> MPPSKGLNGKLEKPKHALQAIVLSDSYNYRFRPLTLDKPRCLLPLANTPLIEYTFEFLALAGVQEVYVFCCAHAGQIREYIEKSKWNLPSSPFSVNTIVSRESLSVGDALRELDSKQLITSDFILVSGDVVSNVPLNEVLKEHRKRREDDKNAIMTMVVREASPFHRTRARTESSVFVIDKKTSQCVHYQANERGKHYVSMDPEIFNEHEELEVRNDLIDCQIDICSNDVPALFTENFDYQDIRKDFVYGVLTSDLLGKKIHCHVAKENYAARVRSLQTYDAISKDVLSRWVYPFVPDSNLLNQTFSYQRHQIYKEEDVVLARSCIIKARTLIGAYTKVG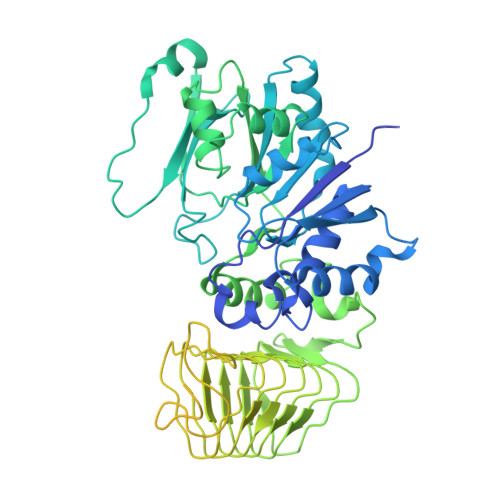DASVVANTIIGRNCTIGSNCSIDSAFLWEDVVIGDNCRIGKAILANSVKIGNNCSIEDGAIVAAGVVIGDNTIIEKNKRLTTFESHSQGTLNDPSLVGIGGRGQEYHAEEDSDDEGEFMEASGLIESTNELHLSDSESSETSSSSEEDMEFIPFSARRDSANTINSEDFDEGDFNKEAQQSLERAFEENHQIDIAALELNTLRMAMNANYHEVRSAIVLALLRRIMHLDVSPKEALAKVMTRWGPLLAKLTFSHEEQVDNVLTLQKYCVRLSMTRHFLQLLGYFYQLEIAEENAIQEWYSDPRSSEGELAALRDAGGKQFVDWLNTAESESESEEGSE N-methyl-5-[(methylamino)methyl]furan-2-carboxamide | C8 H12 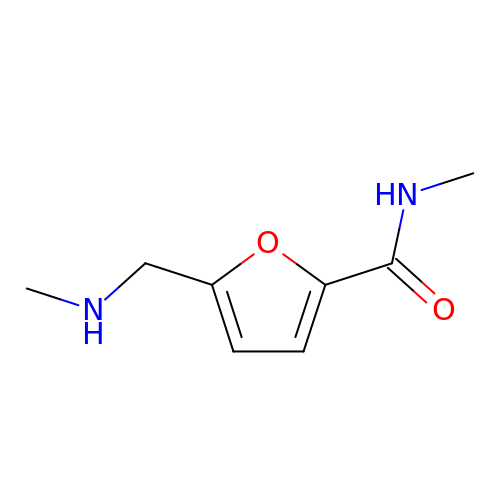N2 O2 | NMODYIFATKWVQB-UHFFFAOYSA-N>MPEIITPIITPFTKDNRIDKEKLKIHAENLIRKGIDKLFVNGTTGLGPSLSPEEKLENLK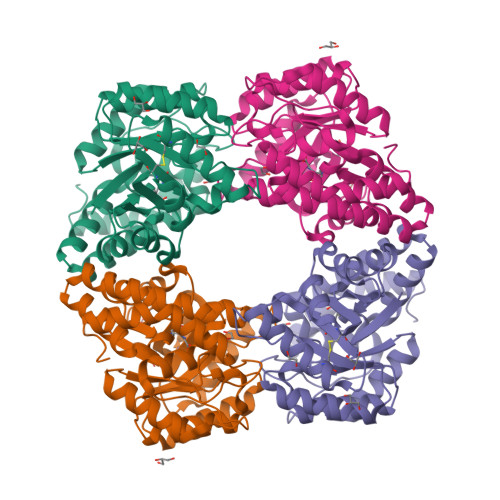AVYDVTNKIIFQVGGLNLDDAIRLAKLSKDFDIVGIASYAPYFYPRMSEKHLVKYFKTLCEVSPHPVYLFNYPTATGKDIDAKVAKEIGCFTGVKDTIENIIHTLDYKRLNPNMLVYSGSDMLIATVASTGLDGNVAFGSNYLPEVTVTIKKLAMERKIDEALKLQFLHDEVIEASRIFGSLSSNYVLTKYFQGYDLGYPRPPIFPLDDEEERQLIKKVEGIRAKLVELKILKE[2x]>ETQPQMFFGVLDREELEYFKQAESTLQLDAFEAPEEKFQFVTSIIEEAKGKELKLVTSQITSKLMERVILECDETQLKDIFQSFNGVFFGLSCHKYASHVLETLFVRSAALVERELLTPSFDNNEKEGPYVTMENMFLFMLNELKPHLKTMMNHQYASHVLRLLILILSSKTLPNSTKANSTLRSKKSKIARKMIDIKDNDDFNKVY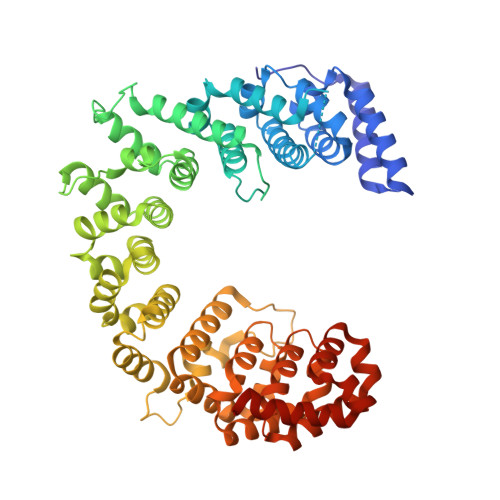QTPESFKSELRDIITTLYKGFTNGAESRSDISQSTITKFREYSVDKVASPVIQLIIQVEGIFDRDRSFWRLVFNTADEKDPKEESFLEYLLSDPVGSHFLENVIGSARLKYVERLYRLYMKDRIVKLAKRDTTGAFVVRALLEHLKEKDVKQILDAVVPELSMLLNSNMDFGTAIINTSNKQGGYLRDDVIAQLIQKYYPEKSDAKNILESCLLLSASTLGNTRDDWPTAEERRRSVFLEQLIDYDDKFLNITIDSMLALPEERLIQMCYHGVFSHVVEHVLQTTRVDIIKRKMLLNILSKESVNLACNVYGSHIMDKLWEFTAKLTLYKERIARALVLETEKVKNSIYGRQVWKNWKLELYVRKMWDWKKLIKEQEFEIFPNSKPLQPKPEK[2x]>[2x]LTLGLAPALSTHSSGVSTQSVDLSQIKRGD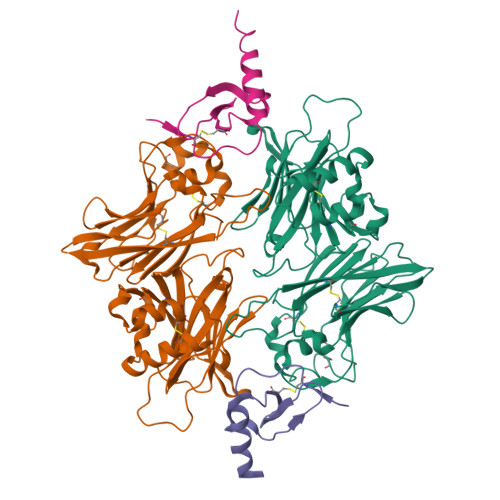EIQAHCLTPAETEVTECAGILKDVLSKNLHELQGLCNVKNKMGVPWVSVEELGQEIITGRLPFPSVGGTPVNDLVRVLVVAESNTPEETPEEEFYAYVELQTELYTFGLSDDNVVFTSDYMTVWMIDIPKSYVDVGMLTRATFLEQWPGAKVTVMIPYSSTFTWCGELGAISEESAPQPSLSARSPVCKNSARYSTSKFCEVDGCTAETGMEKMSLLTPFGGPPQQAKMNTCPCYYKYSVSPLPAMDHLILADLAGLDSLTSPVYVMAAYFDSTHENPVRPSSKLYHCALQMTSHDGVWTSTSSEQCPIRLVEGQSQNVLQVRVAPTSMPNLVGVSLMLEGQQYRLEYFGDH;>VGSEVSDKRTCVSLTTQRLPVSRIKTYTITEGSLRAVIFITKRGLKVCADPQATWVRDVVRSMDRKSNTRNNMIQTKPTGTQQSTNTAVTLTG[2x]>[3x]SNSSFKGSDLPELFSKLGLGKYTDVFQQQEIDLQTFLTLTDQDLKELGITTFGARE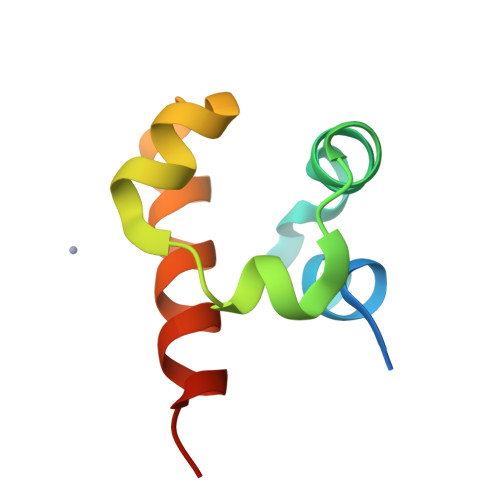KMLLAISELNKNRRK>[2x]GSHMAKEEIIWESLSVDVGSQGNPGIVEY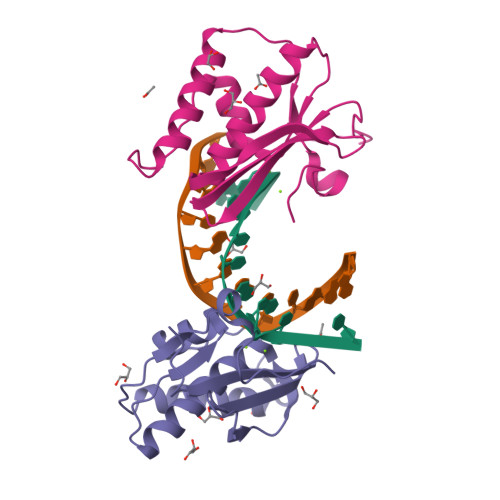KGVDTKTGEVLFEREPIPIGTNNMGEFLAIVHGLRYLKERNSRKPIYSNSQTAIKWVKDKKAKSTLVRNEETALIWKLVDEAEEWLNTHTYETPILKWQTDKWGEIKADYGRK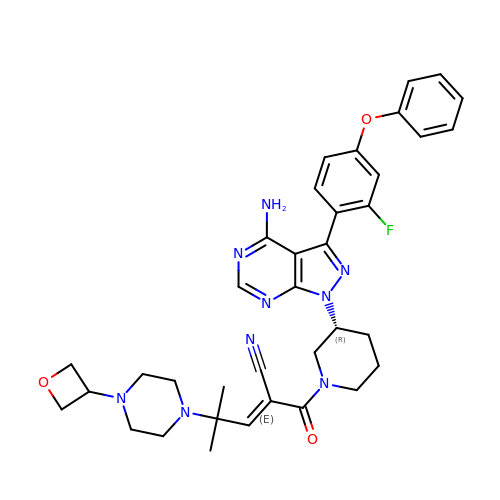(2E)-2-{(3R)-3-[4-amino-3-(2-fluoro-4-phenoxyphenyl)-1H-pyrazolo[3,4-d]pyrimidin-1-yl]piperidine-1-carbonyl}-4-methyl-4-[4-(oxetan-3-yl)piperazin-1-yl]pent-2-enenitrile | C36 H40 F N9 O3 | LCFFREMLXLZNHE-GBOLQPHISA-N>GSAMASNAVLYKSNHNVVYSCKYHIVWCPKYRRKVLVGAVEMRLKEIIQEVAKELRVEIIEMQTDKDHIHILADIDPSFGVMKFIKTAKGRSSRILRQEFNHLKTKLPTLWTNSCFISTVGGAPLNVVKQYIENQQNSN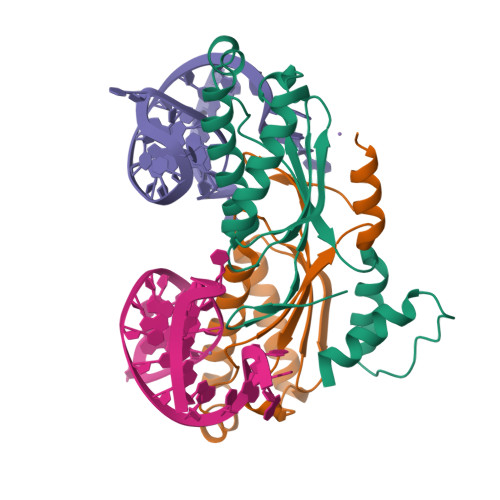RPKQKEKWKSYVDNLQTKAL[2x]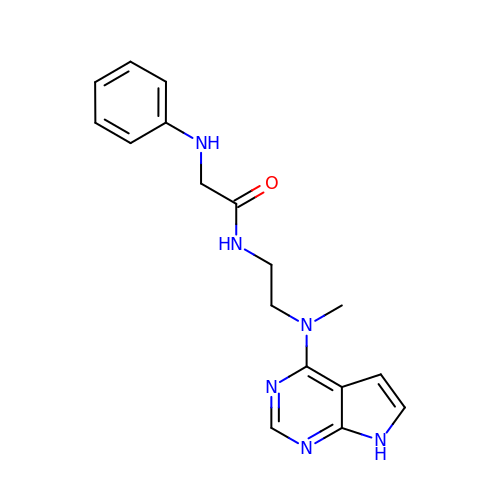N-{2-[methyl(7H-pyrrolo[2,3-d]pyrimidin-4-yl)amino]ethyl}-N~2~-phenylglycinamide | C17 H20 N6 O | IALQDQHYKWZILI-UHFFFAOYSA-N> GSKPRRTKLVFDDRNY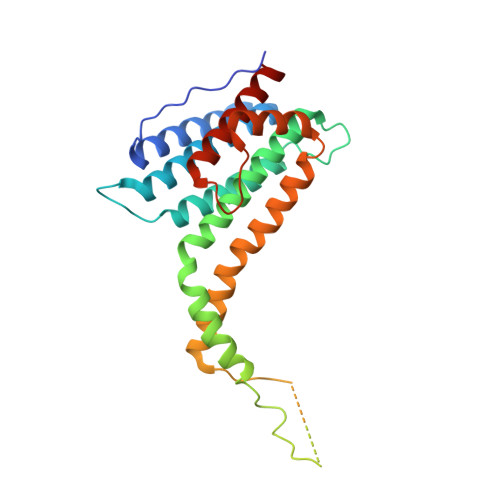SADHYLQEAKKLKHNADALSDRFEKAVYYLDAVVSFIECGNALEKNAQESKSPFPMYSETVDLIKYTMKLKNYLAPDATAADKRLTVLCLRCESLLYLRLFKLKKENALKYSKTLTEHLKNSYNNSQAPSPGLGSKAVGMPSPVSPKLSPGNSGNYSSGASSASASGSSVTIPQKIHQMAASYVQVTSNFLYATEIWDQAEQLSKEQKEFFAELDKVMGPLIFNASIMTDLVRYTRQGLHWLRQDAKLIS> SLKTTREFAGLVLGYDPETGIATVQQRNHFRPGDEVEFF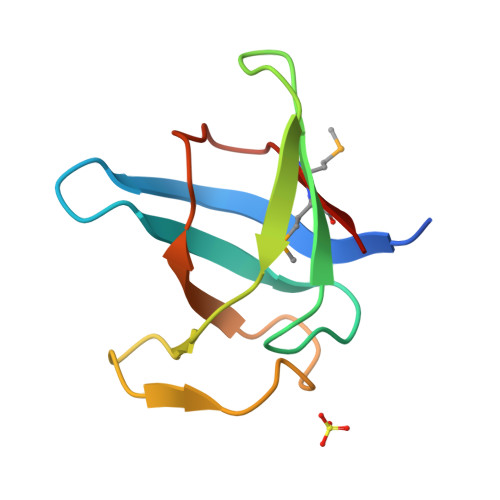GPEIENFTQVIEKIWDEDGNELDAARHPLQIVKFKVKRPLFPYNMMRKEN>QKPGETKEVHPQLTTFRCTKRGGCKPATNFIVLDSLSHPIHRAEGLGPGGCGDWGNPPPKDVCPDVESCAKNCIMEGIPDYSQYGVTTNGTSLRLQHILPDGRVPSPRVYLLDKTKRRYEMLHLTGFEFTFDVDATKLPCGMNSALYLSEMHPTGAKSKYNPGGAYYGTGYCDAQCFVTPFINGLGNIEGKGSCCNEMDIWEANSRASHVAPHTCNKKGLYLCEGEECAFEGVCDKNGCGWNNYRVNVTDYYGRGEEFKVNTLKPFTVVTQFLANRRGKLEKIHRFYVQDGKVIESFYTNKEGVPYTNMIDDEFCEATGSRKYMELGATQGMGEALTRGMVLAMSIWWDQGGNMEWLDHGEAGPCAKGEGAPSN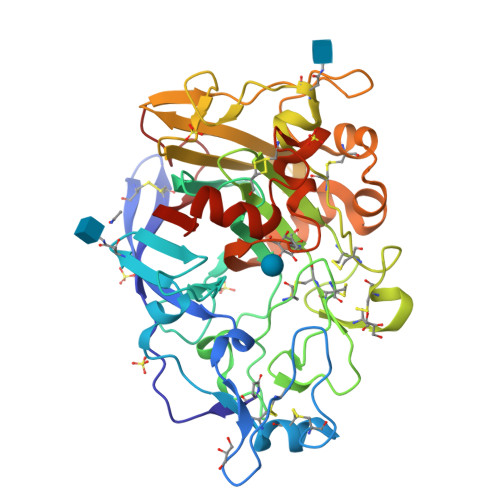IVQVEPFPEVTYTNLRWGEIGSTYQE[2x]>[2x]DSNFPLPDLCSW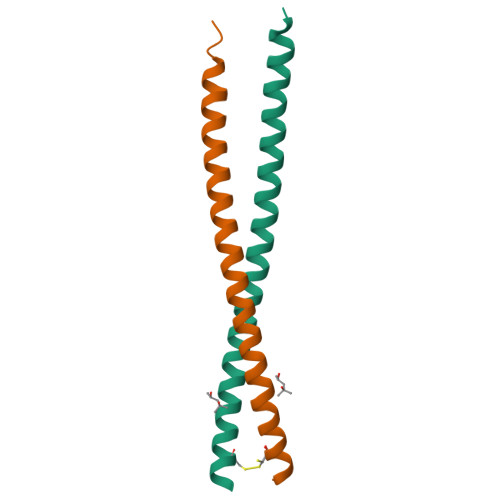EEAQLSSQLYRNKQLQDTLVQKEEELARLHEENNHLRQYLNSALVKCEEEKAKKELSSDEFSKAYGKFRKGKR> MGSSHHHHHHSSGENLYFQGHMTQQPQAKYRHDYRAPDYQITDIDLTFDLDAQKTVVTAVSQAVRHGASDAPLRLNGEDLKLVSVHINDEPWTAWKEEEGALVISNLPERFTLKIINEISPAANTALEGLYQSGDALCTQCEAEGFRHITYYLDRPDVLARFTTKIIADKIKYPFLLSNGNRVAQGELENGRHWVQWQDPFPKPCYLFALVAGDFDVLRDTFTTRSGREVALELYVDRGNLDRAPWAMTSLKNSMKWDEERFGLEYDLDIYMIVAVDFFNMGAMENKGLNIFN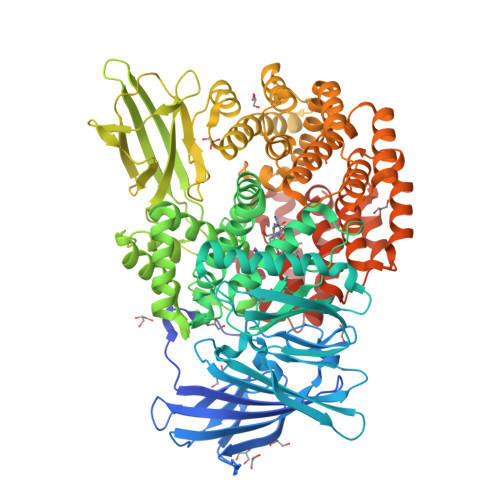SKYVLARTDTATDKDYLDIERVIGHAYFHNWTGNRVTCRDWFQLSLKEGLTVFRDQEFSSDLGSRAVNRINNVRTMRGLQFAEDASPMAHPIRPDMVIEMNNFYTLTVYEKGAEVIRMIHTLLGEENFQKGMQLYFERHDGSAATCDDFVQAMEDASNVDLSHFRRWYSQSGTPIVTVKDDYNPETEQYTLTISQRTPATPDQAEKQPLHIPFAIELYDNEGKVIPLQKGGHPVNSVLNVTQAEQTFVFDNVYFQPVPALLCEFSAPVKLEYKWSDQQLTFLMRHARNDFSRWDAAQSLLATYIKLNVARHQQGQPLSLPVHVADAFRAVLLDEKIDPALAAEILTLPSVNEMAELFDIIDPIAIAEVREALTRTLATELADELLAIYNANYQSEYRVEHEDIAKRTLRNACLRFLAFGETHLADVLVSKQFHEANNMTDALAALSAAVAAQLPCRDALMQEYDDKWHQNGLVMDKWFILQATSPAANVLETVRGLLQHRSFTMSNPNRIRSLIGAFAGSNPAAFHAEDGSGYLFLVEMLTDLNSRNPQVASRLIEPLIRLKRYDAKRQEKMRAALEQLKGLENLSGDLYEKITKALA>[2x]MAHHHHHHMTELRPFYEESQSIYDVSDEFFSLFLDPTMAYTCAY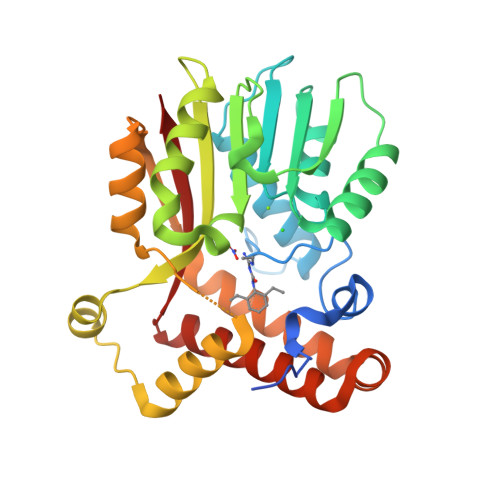FEREDMTLEEAQNAKFDLALDKLHLEPGMTLLDIGCGWGGGLQRAIENYDVNVIGITLSRNQFEYSKAKLAKIPTERSVQVRLQGWDEFTDKVDRIVSIGAFEAFKMERYAAFFERSYDILPDDGRMLLHTILTYTQKQMHEMGVKVTMSDVRFMKFIGEEIFPGGQLPAQEDIFKFAQAADFSVEKVQLLQQHYARTLNIWAANLEANKDRAIALQSEEIYNKYMHYLTGCEHFFRKGISNVGQFTLTK>[6x]PNGDQAARAILIERNLRLVVYIARKFENTGINIEDLISIGTIGLIKAVN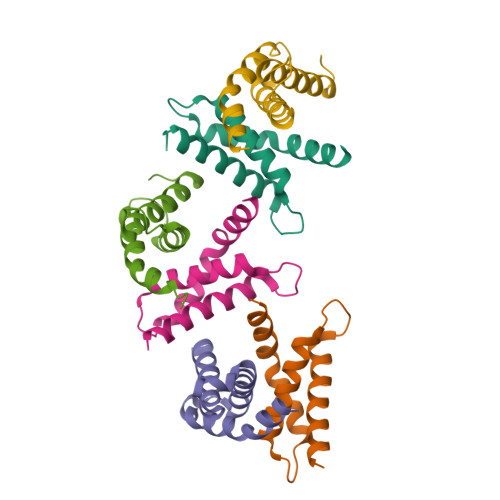TFNPEKKIKLATYASRCIENEILMYLRRNNKIR>[2x]MNDVNRIRTDIINVAKTFGAEYSEKVLDEVFQVFGEQFADNSFMIRTSNKQPDKLGCYFRYHEEDESQLGLAWDIARKSGLLSDQGRPVDQLIPEICETFPIMADGVDFDVKHGLAKIWQSIKGVVPVQDAFKLSLPASVTTHSDFLKNHHLDALYAFGIDYHHSSVNLYFDTYHPKHHTSEYYKNLLQDLQFQPPSDELLELLTNNGEIALTFNFASPRIERLCFYLPFLNREAVPQNLLNPLL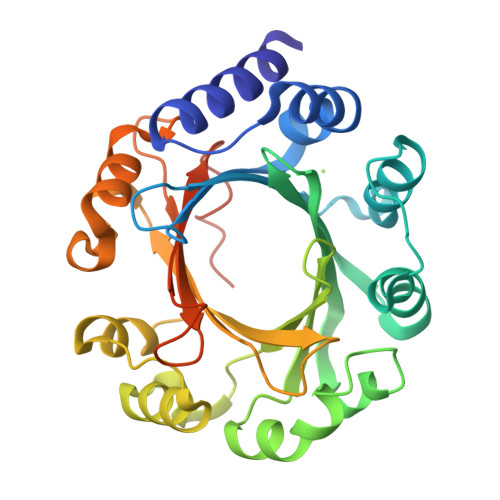KKYINEAPALVDNPGFILGWSFGPQGGKGTYTKVDVDYHGRTVPLFMKVHSQPLPKAADFALAQ>TTVTIVRKDGRIAIAADTLTKWGGGKESADYVANHEKIIRVGDSYVAITGSATFKLILADYFASLDEPPQLDSVARIFCVWNTLHGALKEHYYLQAGEDKEDDLESSRMDVLIANPRGIFGVAAHRTVQEFSKFYAYGSGSPYALGAMYAAYRAPSLDAEAVARLGVMAAAEFHDES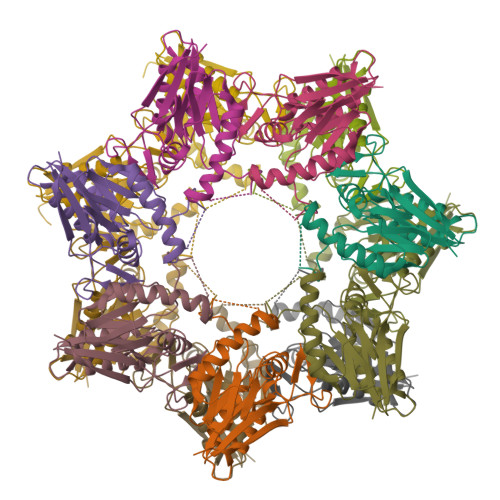GLPVQSFVMELSPDVGSGENLYFQ[14x]>VELIGRSEWINQYRRRLQQLSETDIAVWLYGAPGTGRMTGARYLHQFGRNAQGEFVYRELTPDNAPQLNDFIALAQGGTLVLSHPEHLTREQQYHLVQLQSQEHRPFRLIGIGDTSLVELAASNHIIAELYYCFAMTQIACLPLT[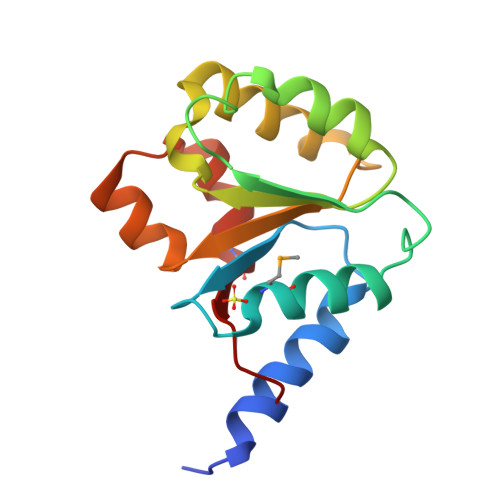8x]SNARE (soluble N-ethylmaleimide-sensitive factor (NSF) attachment protein receptor) proteins drive membrane fusion at different cell compartments as their core domains zipper into a parallel four-helix bundle. After fusion, these bundles are disassembled by the AAA+ (ATPase associated with diverse cellular activities) protein Sec18/NSF and its adaptor Sec17/α-SNAP to make them available for subsequent rounds of membrane fusion. The disassembly requires multiple ATP hydrolysis events in the presence of Mg2+; as few as six ATP hydrolysis events are sufficient. The side-loading and side-release mechanism explains how Sec18/NSF can disassemble SNAREs with constrained topologies.

Next, we asked whether this same side opening of Sec18 occurs in the hydrolyzing condition without SNARE substrate. We prepared purified wild-type Sec18 in the presence of ATP and Mg2+ in a three-stage procedure that yielded a pure sample used for cryo-EM studies. Two bands were visible in native gels, indicating two oligomeric states. Processing and classification led to three classes, two of which appeared to be heptameric and identical (280,935 particles and 73,253 particles, respectively) and a third class that contained indeterminate density in the D1 ring (70,513 particles). Density for the N domains was not well resolved in any of the classes, presumably because of the conformational flexibility of the N domains without substrate or adaptor present. The substrate-free structures (hexamer and heptamer) are nearly identical (r.m.s.d. = 0.48 Å) to the substrate-released structures. The observed coordinated opening in both D1 and D2 rings in conditions with and without substrate suggests a side-release and side-loading mechanism of substrate. We speculate that the conformations of the split Sec18 observed in these multiple conditions are frequently sampled, enabling a substrate to enter or exit the D1–D2 double ring. Given that this opening is hydrolysis independent and occurs regardless of the presence of substrate, it is likely that Sec18 samples these states upon thermal agitation; subsequently, substrate enters the pore and locks the D1 and D2 rings into an active hexameric form (that is, the 20S/y20S complex), possibly in concert with N-domain engagement.

>GAHMFKIPGFGKAAANHTPPDMTNMDTRTRHLKVSNCPNNSYALANVAAVSPNDFPNNIYIIIDNLFVFTTRHSNDIPPGTIGFNGNQRTWGGWSLNQDVQAKAFDLFKYSGKQSYLGSIDIDISFRARGKAVSTVFDQDELAKQFVRCYESQIFSPTQYLIMEFQGHFFDLKIRNVQAIDLGDIEPTSAVATGIETKGILTKQTQINFFKGRDGLVNLKSSNSLRPRSNAVIRPDFKFEDLGVGGLDKEFTKIFRRAFASRIFPPSVIEKLGISHVKGLLLYGPPGTGKTLIARKIGTMLNAKEPKIVNGPEILSKYVGSSEENIRNLFKDAEAEYRAKGEESSLHIIIFDELDSVFKQRGSRGDGTGVGDNVVNQLLAKMDGVDQLNNILVIGMTNRKDLIDSALLRPGRFEVQVEIHLPDEKGRLQIFDIQTKKMRENNMMSDDVNLAELAALTKNFSGAEIEGLVKSASSFAINKTVNIGKGATKLNTKDIAKLKVTREDFLNALNDVTPAFGISEEDLKTCVEGGMMLYSERVNSILKNGARYVRQVRESDKSRLVSLLIHGPAGSGKTALAAEIALKSGFPFIRLISPNELSGMSESAKIAYIDNTFRDAYKSPLNILVIDSLETLVDWVPIGPRFSNNILQMLKVALKRKPPQDRRLLIMTTTSAYSVLQQMDILSCFDNEIAVPNMTNLDELNNVMIESNFLDDAGRVKVINELSRSCPNFNVGIKKTLTNIETARHDEDPVNELVELMTQSA[6x]> MPFCTSTPEPEAQSTEQSLTCEGQIISGTSVDASDLVTGNEIGEQQLISGDAYVGAQQTGCLPTSPRFNQTGNVQSMGFKNTNQPEQNFAPGEVMPTDFSIQTPARSAQNRITGNDIAPSGRITGPGMLATGLITGTPEFRHAARELVGSPQPMAMAMAN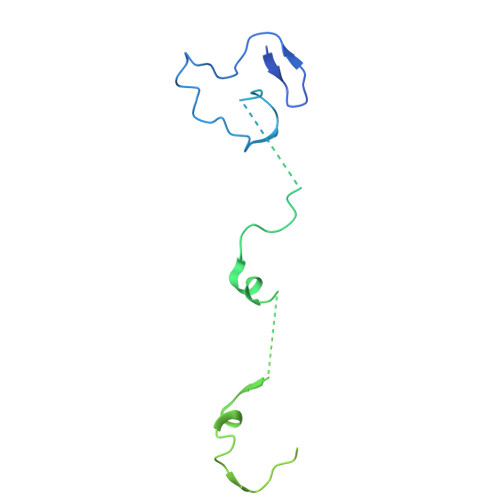RNKAAQAPVVQPEVVATQEKPELVCAPRSDQMDRVSGEGKERCHITGDDWSVNKHITGTAGQWASGRNPSMRGNARVVETSAFANRNVPKPEKPGSKITGSSGNDTQGSLITYSGGARG Thioredoxins (TRX) are small globular proteins of about 100–110 residues, which are conserved in all living organisms. They participate in multiple critical redox-reactions via the reversible oxidation of the active site CXXC catalytic motif1. Two TRX forms were described in Escherichia coli, Trx1 and Trx22. The former, called EcTRX throughout this work, is a widely used experimental model for investigating the molecular basis of protein stability, folding and function.

The N106A variant was designed to eliminate a hydrogen bond linking the side-chain of Asn106 with the carbonyl oxygen of Phe102, thus N106A is expected to destabilize the native structure. The three-dimensional structure of this variant reveals that the hydrogen bond partner of Phe102 is now the main-chain of residue 106, through its amide nitrogen. A slight distortion of the main-chain of the CTH is produced to satisfy the hydrogen bond distance for this interaction. These results are consistent with the very low effect on global stability (ΔΔG°NU = 0.3 kcal mol−1) observed for this mutation. The N106A mutant exhibits a large cavity of 166 Å2 for chain A or 130 Å2 for chain B. Electron density compatible with an ethanol molecule, used as a precipitant, was detected inside this cavity. More likely, the ethanol molecule establishes a hydrogen bond with Leu94. Therefore, we speculate that this cavity of EcTRX is highly dynamic, in such a way that it connects the protein core with the bulk solvent, allowing the entrance of the ethanol molecule. Another significant difference between wild-type and N106A is the distance between loop elements centered in positions 20 and 83, which results in the wild-type structure in a slightly “open” conformation (for instance, the distance from Cα 20 to Cα 83 is 7.4 and 4.3 Å for wild-type and N106A, respectively). For variant N106A, the drop was a 1:1 mix of protein (10 mg/ml) and reservoir solution (100 mM sodium acetate, 4 mM CuSO4, 25% ethanol, pH 4.25).

>MSDKIIHLTDDSFDTDVLKADGAILVDFWAEWCGPCKMIAPILDEIADEYQGKLTVAKLNIDQNPGTAPKYGIRGIPTLLLFKNGEVAATKVGALSKGQLKEFLDAALA[2x]3-[2-amino-6-(2-methylphenyl)quinolin-3-yl]-N-(3,3-dimethylbutyl)propanamide | C25 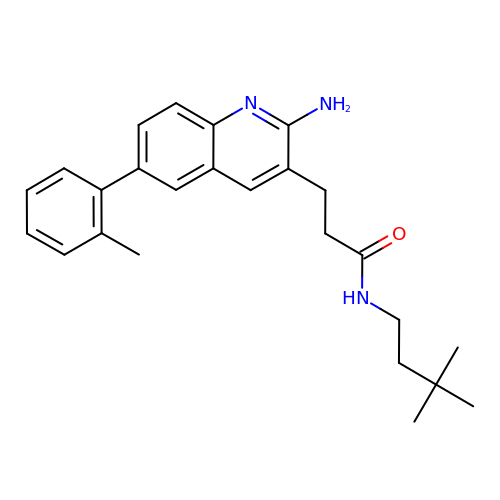H31 N3 O | XKCSLMBNFSFIEK-UHFFFAOYSA-N PANTOTHENYL-AMINOETHANOL-ACETATE PIVALIC ACID | C18 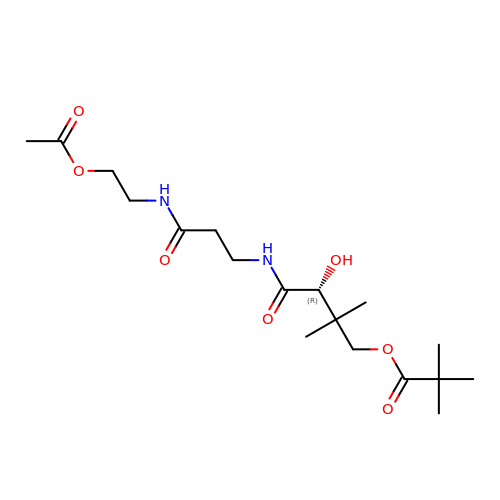H32 N2 O7 | MILJVOHYMMUVQM-AWEZNQCLSA-N The starting point of the engineering efforts reported here is a Kemp eliminase we previously obtained through minimalist design on a β-lactamase background. Our design took advantage of the conformational flexibility of an ancestral β-lactamase scaffold to produce both a suitable cavity and a catalytic base within it through a single mutation, while a second mutation enhanced relevant interactions at the de novo active site. Kemp elimination is a straightforward proton–abstraction reaction that can be performed by a simple molecular machinery consisting, at the bare minimum, of a catalytic base. FuncLib does not per se predict mutations that enhance catalysis, but rather suggests variants with multiple mutations that generate stabilizing interacting networks at the active site, thus focusing the search to safe regions of the sequence space.

Finally, we have used X-ray crystallography to determine the 3D-structures of the catalytically optimized GNCA4-2, GNCA4-12 and GNCA4-19 variants, the first of which has a transition state analogue bound at the de novo active site. These particular structures were chosen as they are all highly active variants, in terms of the measured rates within the available substrate concentration range, with improved catalytic parameters over GNCA4-WT. The protein backbones of these new structures are essentially superimposable with that of the background GNCA4-WT variant and, therefore, the observed enhancement of catalysis is likely linked to small rearrangements in the de novo active site. Here, our crystal structures illustrate that significant gains in activity can be achieved without the need for corresponding significant active site rearrangement. The short extrapolation leads to a catalytic efficiency and a turnover number of about 2 × 104 M–1 s–1 and 102 s–1. These values are well within the ranges of catalytic parameters for modern natural enzymes and, in particular, the value 102 s–1 for kcat is about one order of magnitude higher than the median value of the kcat distribution for modern enzymes. To assess this, we also performed EVB simulations on the variants for which crystal structures were available: GNCA-2, GNCA-12 and GNCA-19. For these variants, the calculated values fall to within 1.3 kcal mol–1 of the experimental values, and can deviate by up to 2.2 kcal mol–1 from the values calculated from the FuncLib predicted structures.

>MAAALSEQLAELEKRSGGRLGVAVLDTATGRRFGYRGDERFPMCSTFKALLAAAVLARVDQGKENLDRRITYGKEDLVDYSPVTEKHVGDGMTVAELCEAAITYSDNTAANLLLEALGGPAALTAFLRSIGDNVTRLDRWEPELNTAAPGDPRDTTTPAAMAATLRTLLLGDVLSPASRQQLVDWLIANKTGDKRLRAGLPADDRVGDKTGTGEHGTTNDIAVVWPPNHAPIFLAVYLTESQVDADARDAVIAEVARLVVAAWVHHHHH[3x]> PNTPWQGYDINTNYYETIPQTNVVREYWFDIVNTTAALDGVERPVLLVNGQFPGPTIEANWGDTVKVHVTNRMENNGTAIHFHGIRQLYNNQMDGVAALTQCPVPPNSSYTYVWRAEEYGSSWYHSHFSLQAWEGVFGGILIHGPSTAEYDHDLGMVFLNDWSHQTVDEMYQSVLESQNPPHFQTGLINGSNIWVTADNQTVGRRFQTEFVPGQRYRLRLVNAAMHTHFRFSIDNHDLTVIASDFVPIVPFTTNNVPIGMGQRYDIIVTANQAPDNYWIRAIPQSFCSDNANSDNIKGVLHYEGAADNSDPTSTKWDYGDDIQCLDFSLDELVPWLALDADIGGAQMAESDVDFTPFGDVPLYLWTMGGNALNISWKDPTLQQTFEDPDK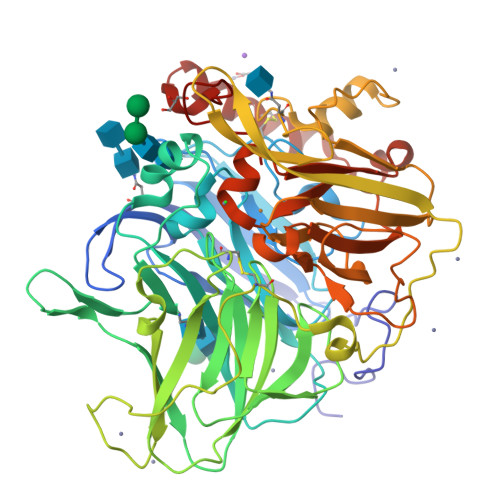MDWKASQGVIEAAIPNKWTVLVVQTDLPVPHPIHLHGHDFYLLAQGFGQFNPQNVTLKTHNPPRRDTALMTAATPENGGGGYMVIGFPADNPGVWLIHCHIGFHATEGFAQQIVERQSEFNTFFSEDLLENTCDAWDEYAKVNPYGHQYRALAGPYESGI>[4x]MAEQTVEAPSVDARAWILMDYASGKVLAEGNADEKLDPASLTKIMTSYVVGQALKADKIKLTDMVTVGKDAWATGNPALRGSSVMFLKPGDQVSVADLNKGVIIQSGNDACIALADYVAGSQESFIGLMNGYAKKLGLTNTTFQTVHG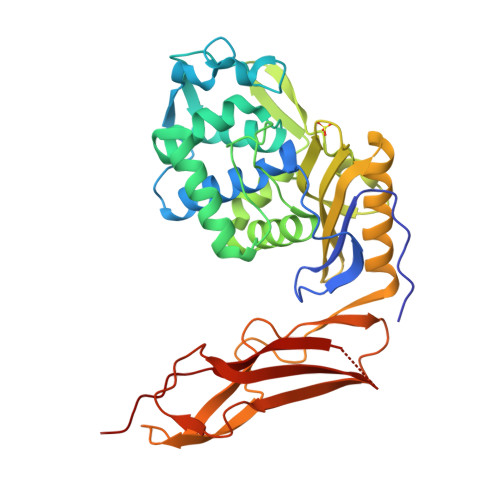LDAPGQFSTARDMALLGKALIHDVPEEYAIHKEKEFTFNKIRQPNRNRLLWSSNLNVDGMKTGTTAGAGYNLVASATQGDMRLISVVLGAKTDRIRFNESEKLLTWGFRFFETVTPIKPDATFVTQRVWFGDKSEVNLGAGEAGSVTIPRGQLKNLKASYTLTEPQLTAPLKKGQVVGTIDFQLNGKSIEQRPLIVMENVEEGG;> AEKAA>MDTTFGLDLARVETLFKRELRRFDELHPRSAQAYRENRRHWLYGAPLHWMQQWPGNCPLLVKEAQGARVTDIDGQQYVDFALGDSGAMFGHAQPAVADAIARQARRGSTLMLPTEDSLWVGAELARRFGLPYWQVTTSATDANRFVLRLCRMLSGRDKVVVFNCNYHGSVDESQVEFDAAGRMVPRAGVHPNGVRHATTTRLVEFNDLDALEAALAHGDVAAVLTEPFMTNVGMVPPAEGFHAGLRELTRRHDVALIIDETHTISCGPAGYSGAHGLEPDFFVLGKCIAGGIPSAVWGCSQAQAERIWAVLPHFRPGQAINHFGFGGTLAGNALQLAAMRATFAEVMTE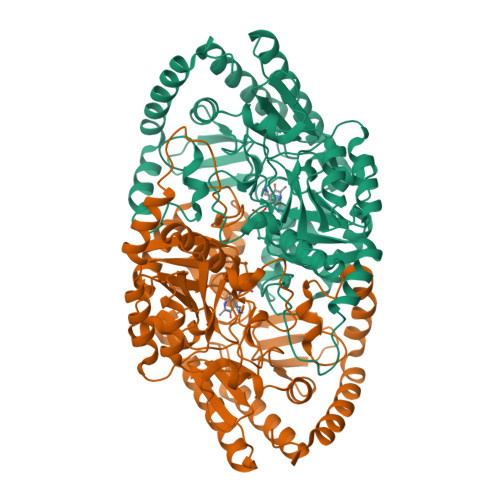DAYRHMFQLAAQLEAGVRATLEELRLPWHVTRIGARVEYLFMTHAPRNGGEAHHARNGLIEACLHLYLLNRGVLLTPFHNMALTCPATRAEDVELHDRLLRDCLGELLERPS[2x]>MYDLLVIGAGPGGYVAAIRAAQLGMKVGVVEKEKALGGTCLRVGCIPSKALLETTERIYEAKKGLLGAKVKGVELDLPALMAHKDKVVQANTQGVEFLFKKNGIARHQGTARFLSERKVLVEETGEELEARYILIATGSAPLIPPWAQVDYERVVTSTEALSFPEVPKRLIVVGGGVIGLELGVVWHRLGAEVIVLEYMDRILPTMDLEVSRAAERVFKKQGLTIRTGVRVTAVVPEAKGARVELEGGEVLEADRVLVAVGRRPYTEGLSLENAGLSTDERGRIPVDEHLRTRVPHIYAIGDVVRGPMLAHKASEEGIAAVEHMVRGFGHVDYQAIPSVVYTHPEIAAVGYTEEELKAQGIPYKVGKFPYSASGRARAMGET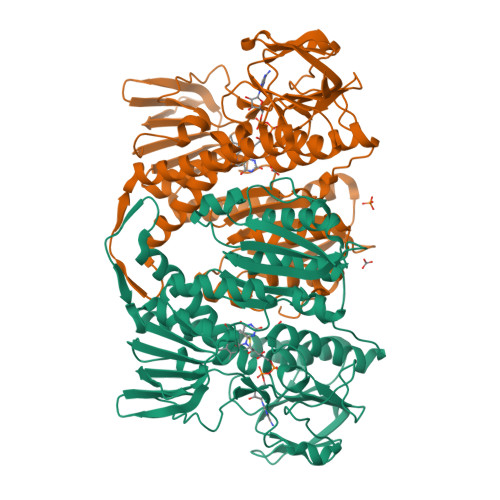EGFIKVLAHAKTDRILGVHGIGARVGDVLAEAALALFFKASAEDLGRAPHAHPSLSEILKEAALAAWERPIHL[2x]>MNPQIRNPMKAMYPGTFYFQFKNLWEANDRNETWLCFTVEGIKRRSVVSWKTGVFRNQVDSETHCHAERCFLSWFCDDILSPNTKYQVTWYTSWSPCPDCAGEVAEFLARHSNVNLTIFTARLYYFQYPCYQEGLRSLSQEGVAVEIMDYEDFKYCWENFVYNDNEPFKPWKGLKTN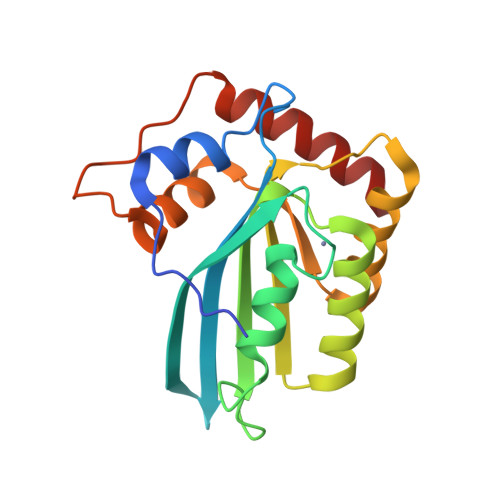FRLLKRRLRESLQ[2x]Glutathione transferases (GSTs) constitute a superfamily of enzymes (EC 2.5.1.18) involved in the metabolism of endogenous and exogenous molecules, widely distributed in nature. They are bisubstratic enzymes mostly known for conjugating GSH to electrophilic molecules, thus increasing their hydrophilicity and facilitating their elimination from the body. Cytosolic GSTs are dimeric enzymes that bear a GSH-binding site (a conserved site known as the G-site) and a binding site for an often-hydrophobic cosubstrate (H-site), in each monomer. Our work shows for the first time that at least two cytosolic hGSTs from different classes, hGST M1-1 and hGST A4-4, catalyze the reaction between NO2-OA and GSH.

To overcome this pitfall, we prepared the GS-10-NO2-OA adduct by mixing a limiting concentration of 10-NO2-OA with excess GSH. hGST M1-1 was crystallized in the presence of the GS-10-NO2-OA adduct and the structure was solved at 2.55 Å resolution. With two dimers in the asymmetric unit, the refined structure displayed the typical features of hGST M1-1, including a conserved N-terminal thioredoxin-like domain (G-site) with typical βαβαββα topology and a C-terminal all-α domain (H-site). Indeed, the GS-10-NO2-OA adduct was bound within the active sites of the four chains within the asymmetric unit, all exhibiting the same binding pose. The electron density map suggested a (R,S) configuration for carbon 20 and carbon 31, respectively, in the four chains of the two homodimers. The glutathionyl portion of the adduct was strongly bound to the protein by many interactions, including several H-bonds and salt bridges, engaging residues Y7, W8, L13, W46, K50, N59, L60, Q72, S73, and D106' (from the other monomer, not shown in the figure). The OH group of Y7, a key residue for catalysis, was at H-bonding distance (3.0 Å) from the sulfur of GS-10-NO2-OA. The fatty acid portion comprising the carbon with the bound nitro group (carbon 31) and the methyl terminus sat in close proximity to the hydrophobic H-site containing nonpolar residues M109, M113, and F209. From the opposite side to Y7, another tyrosine (Y116, on the C-terminal tip of α4) established a 3.3 Å H-bond to one of the oxygens of the fatty acid nitro group. A higher mobility was observed for the carboxylate compared to the rest of the structure, as evidenced by a weaker electron density, as well as higher atomic displacement factors (or B factors). Finally, the crystal structure of hGST M1-1 also suggested that, as there is a fixed and conserved site for GSH binding and a very well-defined site to accommodate and interact with the nitro group, the enzyme can probably only bind and catalyze the reaction using the (E)-isomer of NO2-OA leading to the formation of the product with (R,S) configuration at the chiral carbons 20 and 31, that was observed herein.

>[4x]MPMILGYWDIRGLAHAIRLLLEYTDSSYEEKKYTMGDAPDYDRSQWLNEKFKLGLDFPNLPYLIDGAHKITQSNAILCYIARKHNLCGETEEEKIRVDILENQTMDNHMQLGMICYNPEFEKLKPKYLEELPEKLKLYSEFLGKRPWFAGNKITFVDFLVYDVLDLHRIFEPKCLDAFPNLKDFISRFEGLEKISAYMKSSRFLPRPVFSKMAVWGNK>[6x]MSLTITRIETIPMVAPLAREFRGSHYHMTHRATIVTRVHTDAGIIGEAYTGDEHETMFDIDRIIHEELAPTLIGQDAMAIERLWDSGYKVTFDILRDRRLGLVALAAVNTAIWDAVGKALKMPLWKLWGGYRNELPMIAIGGYYGEPLGSIADEMHNYQELGLAGVKFKVGGLSAAED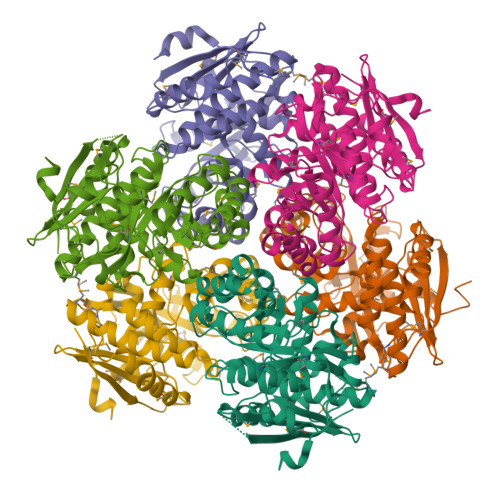AARITAAREAAGDDFIICIDANQGYKPAVAVDLSRRIADLNIRWFEEPVEWHNDKRSMRDVRYQGSVPVCAGQTEFSASGCRDLMETGAIDVCNFDSSWSGGPTAWLRTAAIATSYDVQMGHHEEPQVSTHLLASQPHGTIAECFHPDRDPFWWNMITNRPKLNNGTLTLSDRPGLGWDLNWDYIDQYRVSKDEGHHHHHH> MTHQTHTIAESNNFIVLDKYIKAEPTGDSYQSESDLERELIQDLRNQGYEFISVKSQSAMLANVREQLQNLNGVVFNDSEWRRFTEQYLDNPSDGILDKTRKIHIDYICDFIFDDERLENIYLIDKKNLMRNKVQIIQQFEQAGSHANRYDVTILVNGLPLVQIELKKRGVAIREAFNQIHRYSKESFNSENS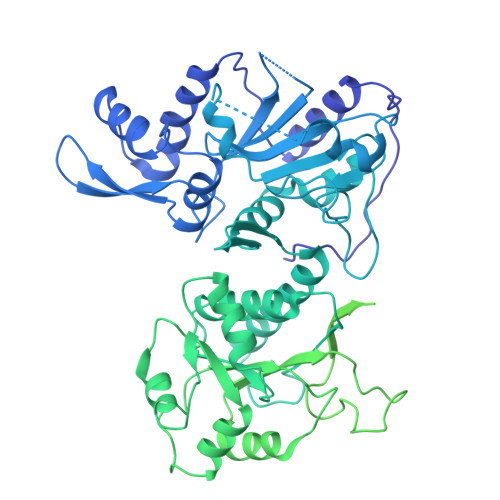LFKYLQLFVISNGTDTRYFANTTKRDKNSFDFTMNWAKSDNTLIKDLKDFTATCFQKHTLLNVLVNYSVFDSSQTLLVMRPYQIAATERILWKIKSSFTAKNWSKPESGGYIWHTTGSGKTLTSFKAARLATELDFIDKVFFVVDRKDLDYQTMKEYQRFSPDSVNGSENTAGLKRNLDKDDNKIIVTTIQKLNNLMKAESDLPVYNQQVVFIFDECHRSQFGEAQKNLKKKFKRYYQFGFTGTPIFPENALGSETTASVFGRELHSYVITDAIRDEKVLKFKVDYNDVRPQFKSLETETDEKKLSAAENQQAFLHPMRIQEITQYILNNFRQKTHRTFPGSKGFNAMLAVSSVDAAKAYYATFKRLQEEAANKSATYKPLRIATIFSFAANEEQNAIGEISDETFDTSAMDSSAKEFLDAAIREYNSHFKTNFSTDSNGFQNYYRDLAQRVKNQDIDLLIVVGMFLTGFDAPTLNTLFVDKNLRYHGLMQAFSRTNRIYDATKTFGNIVTFRDLERSTIDAITLFGDKNTKNVVLEKSYTEYMEGFTDAATGEAKRGFMTVVSELEQRFPDPTSIESEKEKKDFVKLFGEYLRAENILQNYDEFATLKALQQIDLSDPVAVEKFKAEHYVDDEKFAELQTIRLPADRKIQDYRSAYNDIRDWQRREKEAEKKEKSTTDWDDVVFEVDLLKSQEINLDYILGLIFEHNRQNKGKGEMIEEVKRLIRSSLGNRAKEGLVVDFIQQTNLDDLPDKASIIDAFFTFAQREQQREAEALIKEENLNEDAAKRYIRTSLKREYATENGTELNETLPKLSPLNPQYKTKKQAVFQKIVSFIEKFKGVGGKI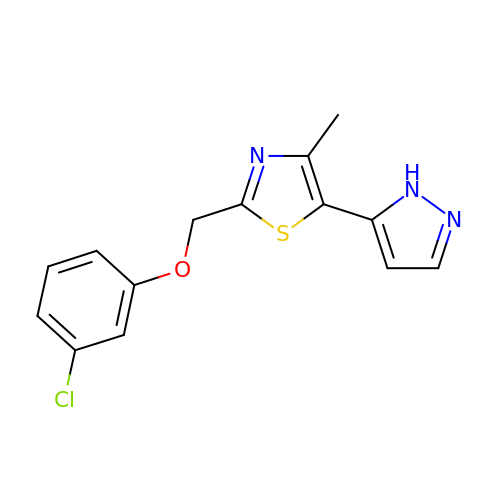2-[(3-chloranylphenoxy)methyl]-4-methyl-5-(1~{H}-pyrazol-5-yl)-1,3-thiazole | C14 H12 Cl N3 O S | NTAUPEMIWLSANJ-UHFFFAOYSA-N>MKYDTSELCDIYQEDVNVVEPLFSNFGGRASFGGQIITVKCFEDNGLLYDLLEQNGRGRVLVVDGGGSVRRALVDAELARLAVQNEWEGLVIYGAVRQVDDLEELDIGIQAMAAIPVGAAGEGIGESDVRVNFGGVTFFSGDHLYADNTGIILSEDPLDIE[3x];> RK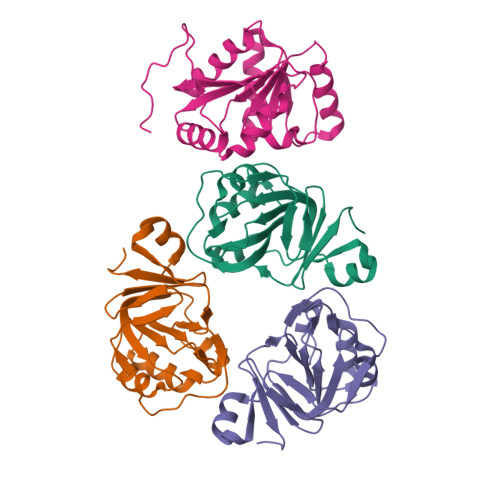KIHQWYYRADDLEHKTALLVHLLKQPEATRSIVFVRKRERVHELANWLREAGINNCYLEGEMVQGKRNEAIKRLTEGRVNVLVATDVAARGIDIPDVSHVFNFDMPRSGDTYLHRIGRTARAGRKGTAISLVEAHDHLLLGKVGRYIEEPIKARVIDELRPKTRAPSE> MQLTPREVEKLMIYTLSDVAFKRKARGLKLNYPEAVSIITVTAMEGARDGKSVEDVMKEASKVLTKDDVMDGVADLIPN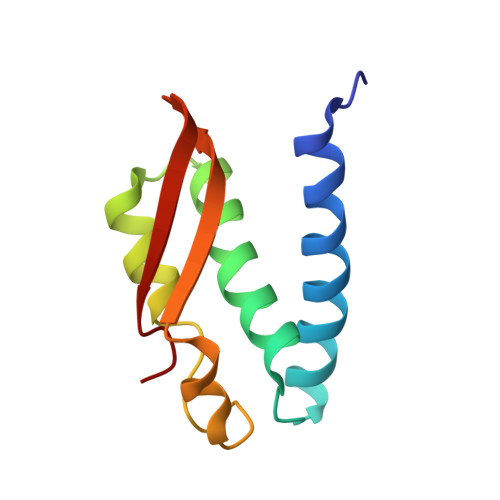VQVEAIFTDGSRLVTVHDPIK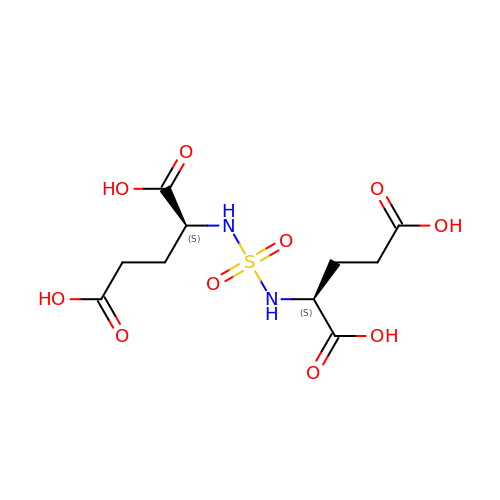(2~{S})-2-[[(2~{S})-1,5-bis(oxidanyl)-1,5-bis(oxidanylidene)pentan-2-yl]sulfamoylamino]pentanedioic acid | C10 H16 N2 O10 S | VLYWUCXOEFVQPS-WDSKDSINSA-N>[2x]GIDPFTMGVITSESEYVSSLSAEKLYRGIVEDGNIIYPKALPRFIEKAE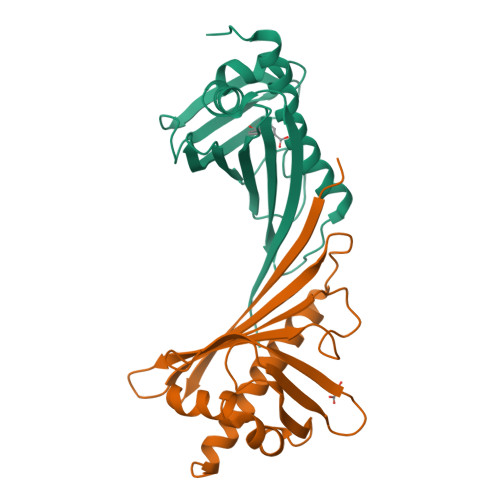TLEGDGGPGTIKKLTFVGDFGSTKQHIDMVDRENCAYTYSVYEGIALSDQPLEKIVFEFKLVPTPEEGCIVKSTTKYYTKGDDIELSKDYLEAGIERFEGFTKAVESFLLANPDYNKDSN>[6x]APQDPRNLPIRQQMEALIRRKQAEITQGLESIDTVKFHADTWTRGNDGGGGTSMVIQDGTTFEKGGVNVSVVYGQLSPAAVSAMKADHKNLRLPEDPKTGLPVTDGVKFFACGLSMVIHPVNPHAPTTHLNYRYFETWNQDGTPQTWWFGGGADLTPSYLYE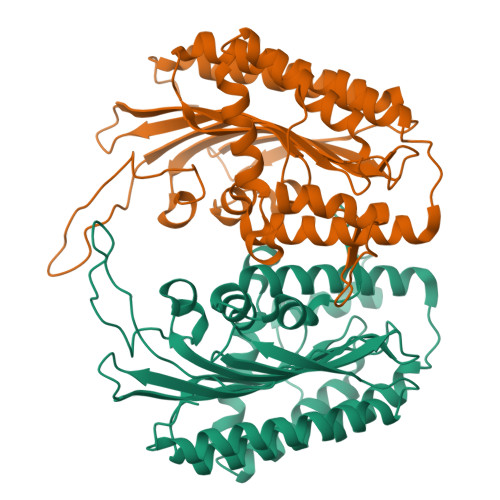EDGQLFHQLHKDALDKHDTALYPRFKKWCDEYFYITHRKETRGIGGIFFDDYDERDPQEILKMVEDCFDAFLPSYLTIVKRRKDMPYTKEEQQWQAIRRGRYVEFNLIYDRGTQFGLRTPGSRVESILMSLPEHASWLYNHHPAPGSREAKLLEVTTKPREWVK> MASMTGGQQMGRGSGSPGVEQHTQAFLEALEQGGGKPLEQLSPKDARAVLTGAQASVKVDLSGIEVKERTIQANGQSIKLQVVRPANVKGELPVFMFFHGGGWVLGDFPTHQRLIRDLVVGSGAVAVYVDYTPSPESHYPTAINQAYAATQWVAEHGKEIGVDGKRLAVAGNAVGGNMAAVVALKAKEAGTPALRFQLLLHPVTDASFETASYKQFADGHFLTTGMMKWFWDNYTTDAKAREQIYASPLRASSEQLKGLPPALVQTAEFDVLRDEGEA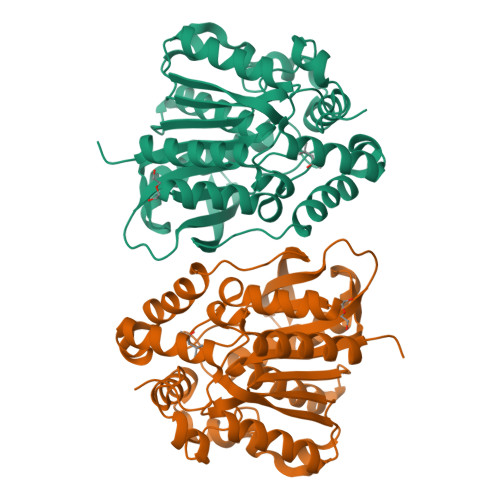YARKLNAAGVTVTSVRYNGMIHDYGLLNPLSQVPAVKAAMRQAGTELKVHLQLEHHHHHH> MLEQPYLDLAKKVLDEGHFKPDRTHTGTYSIFGHQMRFDLSKGFPLLTTKKVPFGLIKSELLWFLHGDTNIRFLLQHRNHIWDEWAF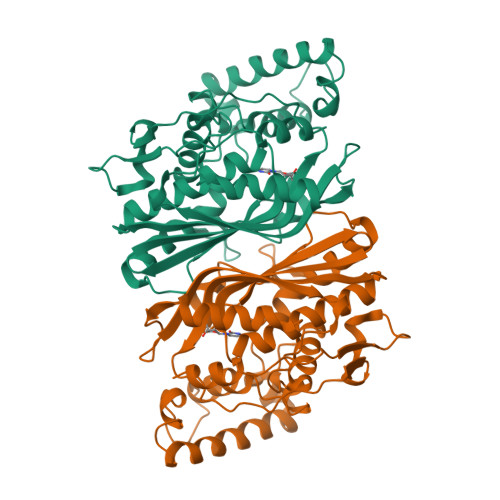EKWVKSDEYHGPDMTDFGHRSQKDPEFAAVYHEEMAKFDDRVLHDDAFAAKYGDLGLVYGSQWRAWHTSKGDTIDQLGDVIEQIKTHPYSRRLIVSAWNPEDVPTMALPPCHTLYQFYVNDGKLSLQLYQRSADIFLGVPFNIASYALLTHLVAHECGLEVGEFIHTFGDAHLWVNHLDQIKEQLSRTPRPAPTLQLNPDKHDIFDFDMKDIKLLNYDPYPAIKAPVAV>[2x]GPNANPIPEHFFAPYIDMSLSVHKPLVEYAKLTGTKYFTLAFILYSSVYNGPAWAGSIPLEKFVDEVRELREIGGEVIIAFGGAVGPYLCQQASTPEQLAEWYIKVIDTYNATYLDFAIEAGIDADKLADALLIVQRERPWVKFSFTLPSDPGIGLAGGYGIIETMAKKGVRVDRVNPMTMDYYWTPSN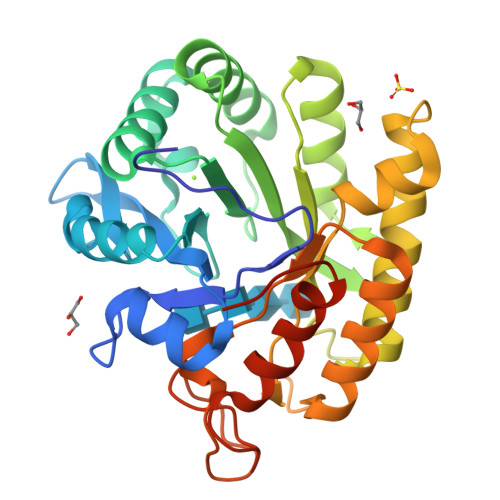AENAIKVAENVFRQLKQIYPEKSDEEIWKMIGLTPMIGVNDDKSVFTLEDAQQLVDWAIQHKIGSLAFWSVDRDHPGPTGEVSPLHRGTNDPDWAFSHVFVKFMEAFGYTFSAQTSEASVPT> QSNAMRLPYSWLREVVAVGASGWDVTPGELEQTLLRIGHEVEEVIPLGPVDGPVTVGRVADIEELTGYKKPIRACAVDIGDRQYREIICGATNFAVGDLVVVALPGATLPGGFTISARKAYGRNSDGMICSAAELNLGADHSGILVLPPGAAEPGADGAGVLGLDDVVFHLAITPDRGYCMSVRGLARELACAYDLDFVDPASNSRVPPLPIEGPAWPLTVQPETGVRRFALRPVIGIDPAAVSPWWLQRRLLLCGIRATCPAVDVTNYVMLELGHPMHAHDRNRISGTLGVRFARSGETAVTLDGIERKLDTADVLIVDDAATAAIGGVMGAASTEVRADSTDVLLEAAIWDPAAVSRTQRRLHLPSEAARRYERTVDPAISVAALDRCARLLADIAGGEVSPTLTDWRGDPPCDDWSPPPIRMGVDVPDRIAGVAYPQGTTARRLAQIGAVVTHDGDTLTVTPPSWRPDLRQPADLVEEVLRLEGLEVIPSVLPPAPAGRGLTAGQQRRRTIGRSLALSGYVEILPTPFLPAGVFDLWGLEADDSRRMTTRVLNPLEADRPQLATTLLPALLEALVRNVSRGLVDVALFAIAQVVQPTEQTRGVGLIPVDRRPTDDEIAMLDASLPRQPQHVAAVLAGLREPRGPWGPGRPVEAADAFEAVRIIARASRVDVTLRPAQYLPWHPGRCAQVFVGESSVGHAGQLHPAVIERSGLPKGTCAVELNLDAIPCSAPLPAPRVSPYPAVFQDVSLVVAADIPAQAVADAVRAGAGDLLEDIALFDVF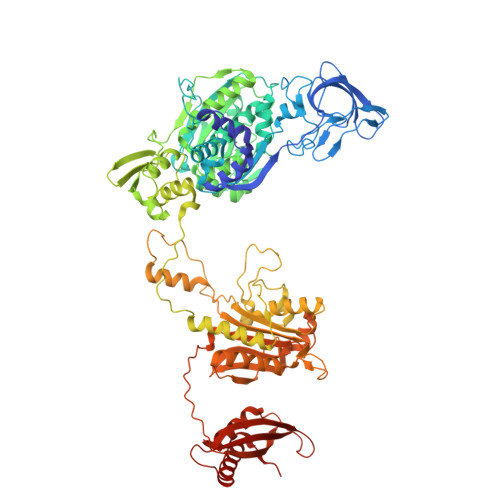TGPQIGEHRKSLTFALRFRAPDRTLTEDDASAARDAAVQSAAERVGAVLRG>SGSGSDDHSSARKFADEFREMMKTGDSTKADELFDPNVRVEVGDKRYHGREQAVDWIRHLVDRYDHIEIRIDHITVRGDRISIVFTVHYEKNGETTYDRYVMVAVDRNG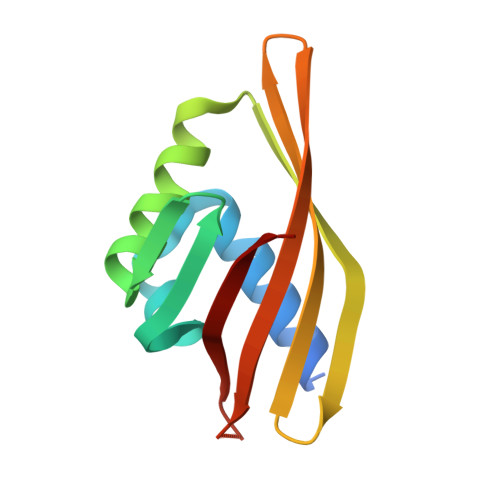RAQIKMLRKG[2x]>[2x]MPEVVGSYFQSNAMTGPHAAGGSNHRTARLVAIIAGLLGTLMAIATPLLPVEQTTAELNWPQNGVWQSVDAPLIGYVATDLTVTVPCQAAAGLVGPENRNRSVLLSTVPKQAPKAIDRGLLIERINNDLTVIVRNTPVVSAPLEQVLSPDCRYLTFTAHADKVTGEFVGLTQGPDDDDPGEAVRGERSGYDFRPQIVGVFTD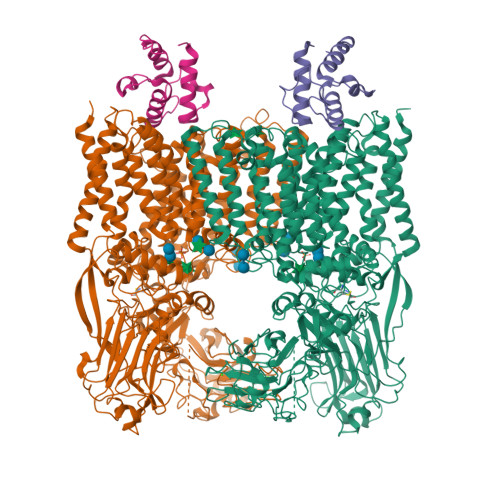LSGPAPEGLQLSATIDTRYSTSPTLLKLLAMIVGVAMTVIALGALHVLDCADGRRHKRFLPSRWWSMTPLDGLVSAMLVWWHFVGANTADDGYILTMARVSEHAGYMANYYRWFGTPESPFGWYYDLLALWAHVSTASVWMRFPTLLMGLACWWVISREVIPRLGAAAKHSRAAAWTAAGLFLAFWLPLNNGLRPEPIIALGILLTWCSVERGVATSRLLPVAVAIIIGALTLFSGPTGIAAVGALLVAIGPLKTIVAAHVSRFGYWALLAPIAAAGTVTIFLIFRDQTLAAELQASSFKSAVGPSLAWFDEHIRYSRLFTTSPDGSVARRFAVLTLLLALAVSIAMTLRKGRIPGTALGPSRRIIGITIISFLAMMFTPTKWTHHFGVFAGLAGCLGALAAVAVTTTAMKSRRNRTVFGAAVLFVTALSFATVNGWWYVSNFGVPWSNSFPEFKFGFTTMLLGLSVLALLVAAWFHFSGRDVSPDRPQRRWQRLLVAPLAVATWALVIFEVVSLTLGMINQYPAWSVGRSNLNALTGKTCGLANDVLVEQNANAGMLTPIGEPAGQALGAVTSLGFGPNGIPSDVSADPVMEQPGTDNFADSDSGVVTGTEVGTEGGTTAAAGINGSRARLPYGLNPATTPVLGSWRSGTQQPAVLRSAWYRLPDRDQAGPLLVVSAAGRFDQGEVEVQWATDEQAAANEPGGSITFGDVGAAPAWRNLRAPLSSIPPEATQIRLVASDDDLAPQHWIALTPPRIPELRTLQEVVGSSDPVMLDWLVGLAFPCQRPFDHRYGVVEVPKWRILPDRFGAEANSPVMDYLGGGPLGITELLLRPSSVPTYLKDDWYRDWGSLQRLTPWYPDAQPARLDLGTATRSGWWSPAPLRLSHLGGIKAFLEVLFQGPHHHHHHHHHH;>[2x]MAATQEEIIAGLAEIIEEVTGIEPSEVTPEKSFVDDLDIDSLSMVEIAVQTEDKYGVKIPDEDLAGLRTVGDVVAYIQKLEEENPEAAAALREKFAADQ> MKKEVRKVRIALASPEKIRSWSYGEVEKPETINYRTLKPERDGLFDERIFGPIKDYECACGKYKRQRFEAKVCERCAVEVTRSIVRRYRMAHIELATPAAHIWFVKDVPSKIATLLDLSATELEQVLYFNKYIVLDPKAAVLDAVPVEKRQLLTDXXXXXXXXXXXXXXXXXXXXXXXXXXXXXXXXXXXXIDARMGAEAIQELLKELDLEKLERELLEEMKHPSRARRAKARKRLEVVRAFLDSGNRPEWMILEAVPVLPPDLRPMVQVDGGRFATSDLNDLYRRLINRNNRLKKLLAQGAPEIIIRNEKRMLQEAVDAVIDNGRRGSPVTNPGSERPLRSLTDILSGKQGRFRQNLLGKRVDYSGRSVIVVGPQLKLHQCGLPKRMALELFKPFLLKKMEEKAFAPNVKAARRMLERQRDIKDEVWDALEEVIHGKVVLLNRAPTLHRLGIQAFQPVLVEGQSIQLHPLVCEAFNADFDGDQMAVHVPLSSFAQAEARIQMLSAHNLLSPASGEPLAKPSRDIILGLYYITQVRKEKKGAGMAFATPEEALAAYERGEVALNAPIVVAGRETSVGRLKFVFANPDEALLAVAHGLLDLQDTVTTRYLGRRLETSPGRILFARIVGEAVGDEK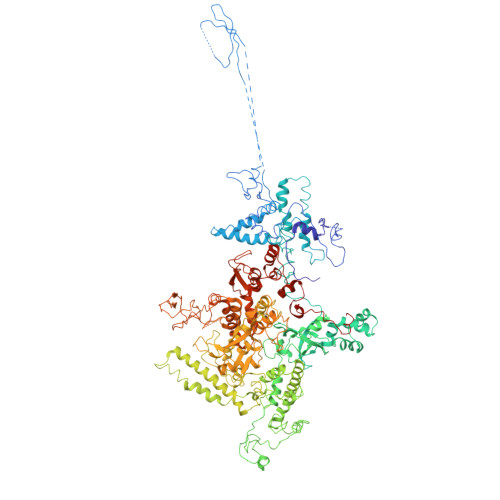VAQELIQMDVPQEKNSLKDLVYQAFLRLGMEKTARLLDALKYYGFTLSTTSGITIGIDDAVIPEEKQRYLEEADRKLRQIEQAYEMGFLTDRERYDQVIQLWTETTEKVTQAVFNNFEENYPFNPLYVMAQSGARGNPQQIRQLCGMRGLMQKPSGETFEVPVRSSFREGLTVLEYFISSHGARKGGADTALRTADSGYLTRKLVDVAHEIVVREADCGTTNYISVPLFQMDEVTRTLRLRKRSDIESGLYGRVLAREVEALGRRLEEGRYLSLEDVHFLIKAAEAGEVREVPVRSPLTCQTRYGVCQKCYGYDLSMARPVSIGEAVGVVAAESIGEPGTQLTMRTFHTGGVAVGTDITQGLPRVIELFEARRPKAKAVISEIDGVVRIEEGEDRLSVFVESEGFSKEYKLPKDARLLVKDGDYVEAGQPLTRGAIDPHQLLEAKGPEAVERYLVDEIQKVYRAQGVKLHDKHIEIVVRQMLKYVEVTDPGDSRLLEGQVLEKWDVEALNERLIAEGKVPVAWKPLLMGVTKSALSTKSWLSAASFQNTTHVLTEAAIAGKKDELIGLKENVILGRLIPAGTGSDFVRFTQVVDQRTLKAIEEARKEAVEAKEKEAPRRPVRREQPGKGL>GIDPFTMSDLPCPPTNAERLHEFHRAIGAATPERPTPPPPELLRLRQTLLDEESAEVRAEIDHLLARQAAGEALSAGDLAPLAHELADLLYVTYGALDQLGIDADAVFAEVHRAN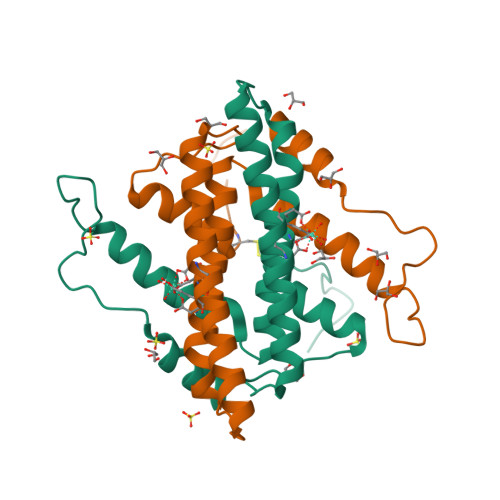LSKASGPRRADGKQLKPEGWRPADVRGVIERLQHAPADD[6x]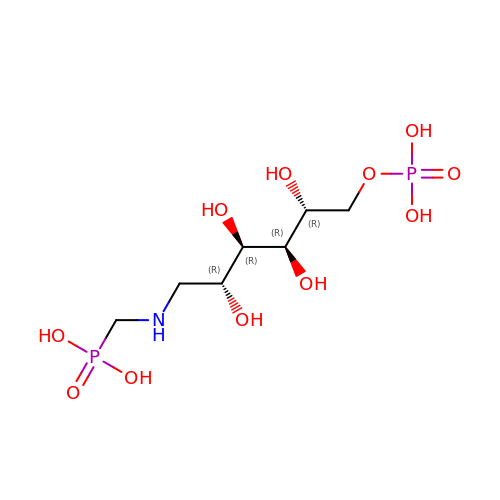1-DEOXY-6-O-PHOSPHONO-1-[(PHOSPHONOMETHYL)AMINO]-L-THREO-HEXITOL | C7 H19 N O11 P2 | YAEYOLVKVWEHNB-DBRKOABJSA-N> MAEEYSWDSYLNDRLLATNQVSGAGLASEEDGVVYACVAQGEESDPNFDKWSLFYKEDYDIEVEDENGTKTTKTINEGQTILVVFN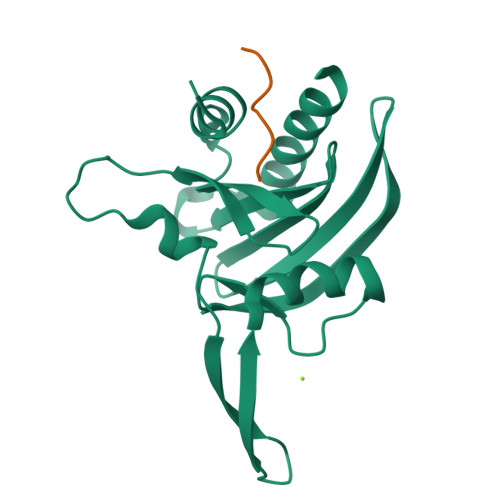EGYAPDGVWLGGTKYQFINIERDLEFEGYNFDVATCAKLKGGLHLVKVPGGNILVVLYDEEKEQDRGNSKIAALTFAKELAESSQLQHHHHHH;> PPPPPPPP> MEGIDMPATNAVRPFGRNYSGGQQQAISRFTARPGDPQVEELYLIFTNFPAQTAYWEFHKKVLACAIRLFSGNYNWFILQDNNSNIDSYNYQFLLDTVRYIATGHRRISIT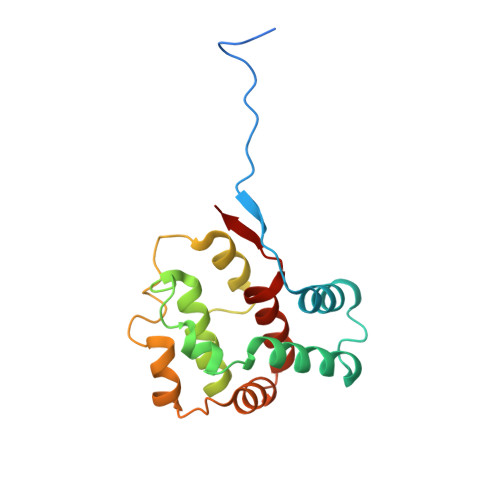QWPMLLATEPDAGAQLIEPRAEIATLFNELKLDLDTVSMIQNWVKHKNGMNDLMYTLHLLFGSVEVIDKD> LVATTSSKIYDNKNQLIADLGSER;> SASNYPAYMDNYLKEVINQVEQETGYNLLTTGMDVYTNVDQEAQKHLWDIYNSDQYVSYPDDDLQVASTVVDVSNGKVIAQLGARHQA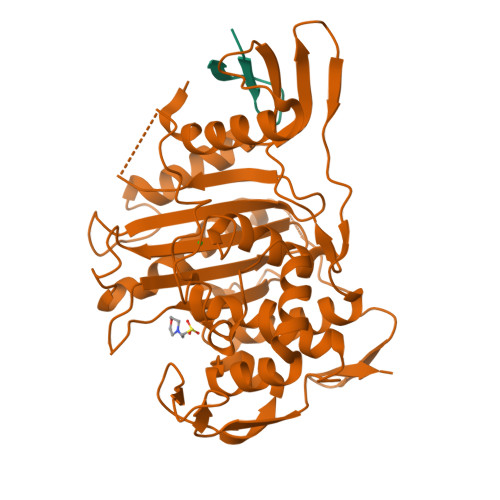SNVSFGTNQAVETNRDWGSAMKPITDYAPAIEYGVYDSTATMVNDIPYNYPGTSTPVYNWDRAYFGNITLQYALQQSRNVTAVETLNKVGLDRAKTFLNGLGIDYPSMHYANAISSNTTESNKQYGASSEKMAAAYAAFANGGIYHKPMYINKVVFSDGSKKEFSDVGTRAMKETTAYMMTEMMKTVLAYGTGRGAYLPWLAQAGKTGTSNYTDDEIEKHIKNTGYVAPDEMFVGYTRKYSMAVWTGYSNRLTPIVGDGFLVAAKVYRSMITYLSEGSNPEDWNIPEGLYRNGEFVFKNGAR2-(2,6-difluorophenyl)-4-[4-(pyrrolidine-1-carbonyl)anilino]-5H-pyrrolo[3,4-b]pyridin-5-one 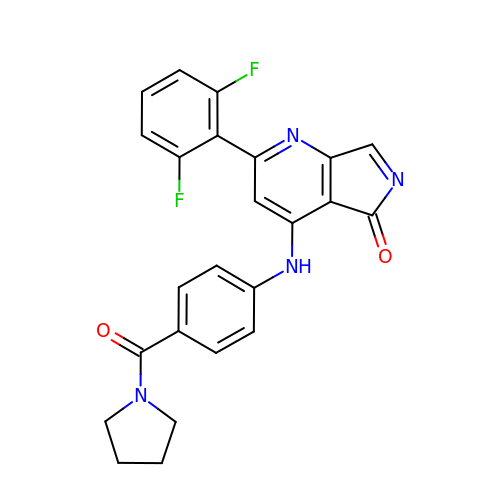| C24 H18 F2 N4 O2 | IIQPGWZFSIWDHM-UHFFFAOYSA-N>IRVFAIPPSFASIFLTKSTKLTCLVTDLTTYDSVTISWTRQNGEAVKTHTNISESHPNATFSAVGEASICEDDWNSGERFTCTVTHTDLPSPLKQTISRPKGVALHRPDVYLLPPAREQLNLRESATITCLVTGFSPADVFVQWMQRGQPLSPEKYVTSAPMPEPQAPGRYFAHSILTVSEEEWNTGETYTCVVAHEALPNRVTERTVDKSTGKPTLYNVSLVMSDTAGTC[10x];> EDERIVLVDNKCKCARITSRIIRSSEDPNEDIVERNIRIIVPLNNRENISDPTSPLRTRFVYHLSDLCKKCDPTEVELDNQIVTATQSNICDEDSATETCYTYDRNKCYTAVVPLVYGGETKMVETALTPDACYPD;>RILPEVKVEGELGGSVTIKCPLPEMHVRIYLCREMAGSGTCGTVVST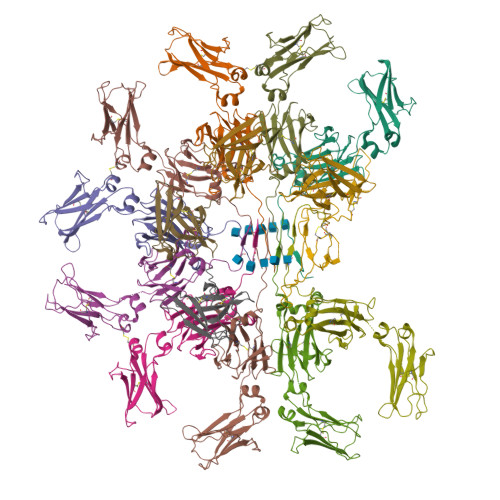TNFIKAEYKGRVTLKQYPRKNLFLVEVTQLTESDSGVYACGAGMNTDRGKTQKVTLNVHS[4x]> GAMESKKRQWALEDFEIGRPLGKGKFGNVYLAREKQSKFILALKVLFKAQLEKAGVEHQLRREVEIQ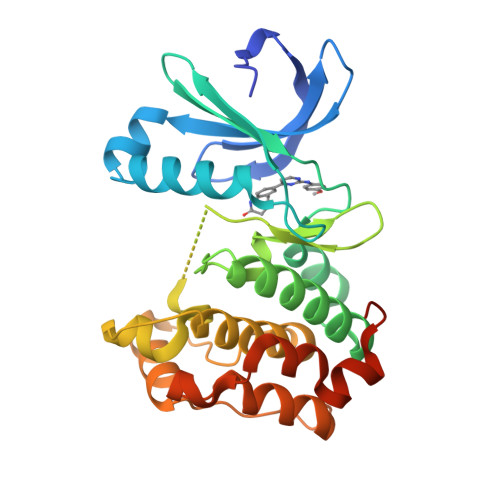SHLRHPNILRLYGYFHDATRVYLILEYAPLGTVYRELQKLSKFDEQRTATYITELANALSYCHSKRVIHRDIKPENLLLGSAGELKIADFGWSVHAPSSRRTTLCGTLDYLPPEMIEGRMHDEKVDLWSLGVLCYEFLVGKPPFEANTYQETYKRISRVEFTFPDFVTEGARDLISRLLKHNPSQRPMLREVLEHPWITANSSKPSNCQNKESASKQS Earlier, we identified dextranase (FjDex31A) and kojibiose hydrolase (FjGH65A) in the dextran utilization locus (FjDexUL) of a soil Bacteroidota Flavobacterium johnsoniae and hypothesized that FjDexUL is involved in the degradation of α-(1→2)-branched dextran. FjDexUL consists of eight genes that encode proteins Fjoh_4428–Fjoh_4435: SusR homolog (Fjoh_4435, hereafter FjDusR), SusC homolog (Fjoh_4434, FjDusC), SusD homolog (Fjoh_4433, FjDusD), SusE/F homolog (Fjoh_4432, FjDusE), GH66 enzyme (Fjoh_4431, FjGH66), GH31 dextranase (Fjoh_4430, FjDex31A), GH97 enzyme (Fjoh_4429, FjGH97A), and GH65 kojibiose hydrolase (Fjoh_4428, FjGH65A). FjDexUL glycoside hydrolases synergistically degraded S-32 α-glucan. Collectively, FjDexUL proteins are suggested to be involved in the degradation of α-(1→2)- and α-(1→3)-branched dextrans.

FjGH65A hydrolyzes the α-(1→2)-glucosidic linkage in kojibiose (α-(1→2)-glucobiose) and longer kojioligosaccharides. FjGH65A showed low activity against S-32 α-glucan and S-64 α-glucan, although it has activity against 6-O-α-kojibiosylglucose, which is a substructure of α-(1→2)-branched dextran, comparable with kojibiose and kojitriose. To clarify how the enzyme recognizes 6-O-α-kojibiosylglucose, the IG2-complex structure was examined. The 1.56-Å resolution structure enabled us to identify distinct electron densities for IG2 at subsites +1 and +2. The glucose residue at the nonreducing end of IG2 at subsite +1 (Glc +1) is recognized by Arg74, Glu392, Trp391, Thr407, and Glu472 (catalytic residue) through hydrogen bonds. The glucose residue at the reducing end at subsite +2 (Glc +2) is recognized by Glu475, Lys538, and the main chain O of catalytic Glu472 through hydrogen bonds. Among the hydroxy groups of Glc +1 of IG2, O2 atom of Glc +1 is the closest to the anomeric C1 atom of glucose at subsite −1 of the glucose complex at a distance of 2.4 Å. The reducing end of IG2 is directed toward the solvent, whereas 6-OH of Glc +1 at the nonreducing end is blocked by Arg74. The structure of FjGH65A in complex with isomaltose supports that FjGH65A acts on α-(1→2)-glucosyl isomaltooligosaccharides. The IG2-complex structure of FjGH65A suggests that FjGH65A can only hydrolyze the α-(1→2)-glucosidic linkage on the nonreducing end but not on the intermediate α-(1→2)-branches in branched dextran.

>[3x]MGSSHHHHHHSSGLVPRGSHQDPWKLSADKPDSNNYYGETVANGMIGIISSPEPLKVKEVVLAGTYDIYKRGRVSSFIPNYNLLNMKLAFNGESVQTYNINNYKQELDMRNGAFTGSFQFKDLATVTYSYYALRHLPHCIMMVVNINTQKDTEINVENLLETPSSLNNQQNYFQNITNTHVNIPLLTSVAFTPTGRSKIAVSNTFLFDEGKKLQPEILHRMNDADMHAMSFDKKIKAGKTYSFALIGSLISSDHINDPYNEAERLTIYAALEGKSRLLNRHMQEWNSLWQSDIQVEGDPQAQQDIRSMLYHLYSFTRKSTSLSPSPMGLSGLGYNGHVFWDTEIWMFPPMLLLHPEIAKSMIEYRYQRLDAARKKAAIYGYDGAMFPWESADSGAEETPVNALTGAFEHHVTGDVAIAAWQYYLVTGDKEWLKEKGWPILKATAEFWASRVEKNDKGEYEIKNVVAADEWAENIDNNAYTNGTAIRNLQYASKCATVLGVIAPKEWTLIADKILISKMSNGVTREHDSYTDQNIKQADANLLAYPLKLITDKEQIERDLKYYQTKIPQSDTPAMTQAIFSLLYSRLEDSDQAYHWFKDAYQPNLNPPFRVISECKGGTNPYFSTGAGGVLQAVIMGFGGLDIDAAGGIKQVKSVLPKNWKKLTITGIGIEKKTFVLTH>MTLDVWQHIRQEAKELAENEPMLASFFHSTILKHQNLG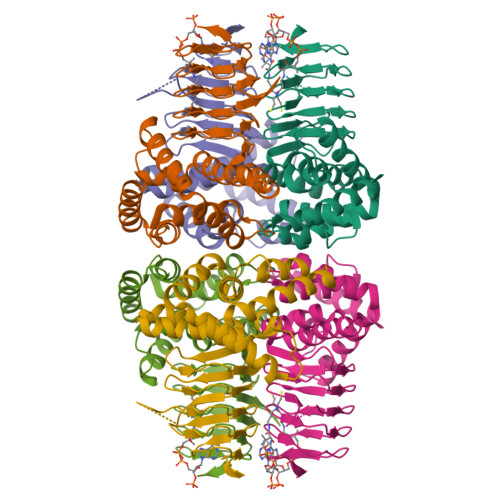GALSYLLANKLANPIMPAISLREIIEEAYQSNPSIIDCAACDIQAVRHRDPAVELWSTPLLYLKGFHAIQSYRITHYLWNQNRKSLALYLQNQISVAFDVDIHPAAKIGHGIMFDHATGIVVGETSVIENDVSILQGVTLGGTGKESGDRHPKVREGVMIGAGAKILGNIEVGKYAKIGANSVVLNPVPEYATAAGVPARIVSQDKAAKPAFDMNQYFIGIDDGMNLNI[3x]>[2x]MKKILVIS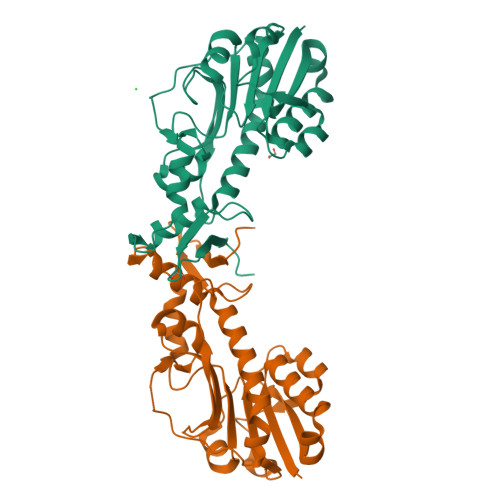DNYQLVSYIKNLYLSNEEWSKELFIDYSYSSINRNPQSLIELGMTEIDIKNKNLNELNDYHLIISAHCKQIFPAHIVNNKLCINIHPGLNPYNRGWFPQVFSILNKKPIGATIHKMDSEVDHGEIYCQEEVSILSHETSIDIYNKVIELEKKLIKNNLLKIINNELQPKLPSQEGNYNSIQDFNKLCKLNLEDNGSLREHIDLLRALTHGDFKNAYFYDENNTKVFVKIELSLSQELESAHHHHHH>GHMTASFPTRVYLLRHAKAAWA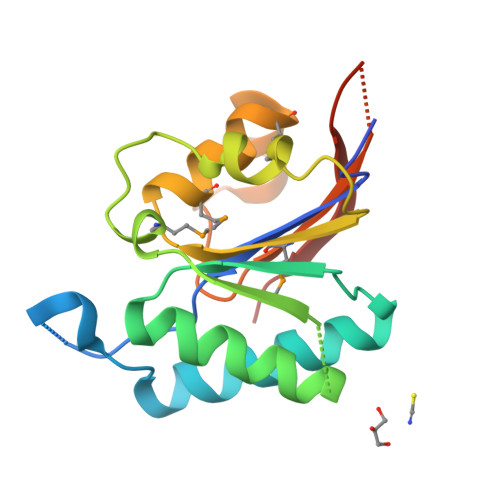APGERDFDRGLNEAGFAEAEIIADLAADRRYRPDLILSSTAARCRQTTQAWQRAFNEGIDIVYIDEMYNARSETYLSLIAAQTEVQSVMLVGHNPTMEATLEAMIGEDLLHAALPSGFPTSGLAVLDQDDSAASGKNRWRLIDFLAPGKGS[8x]> GDNQDRTVANTQPSGPSNSKEIPALTAVETGHTSQVDPSDTLQTRHVVNFHSRSESTVENFMGRAACVFMDQYKLNGEETSTDNFAVWTINVREMAQLRRKCELFTYMRFDIEMTMVITSCQDQGTQLEQDMPVLTHQIMYVPPGGPIPAKVDSYEWQTSTNPSVFWTEGNAPARMSIPFISVGNAYSLFYDGWSHFTQDGTYGYTTLNAMGKLFVRHVNKSSPHQITSTIRVYFKPKHIKAWVPRP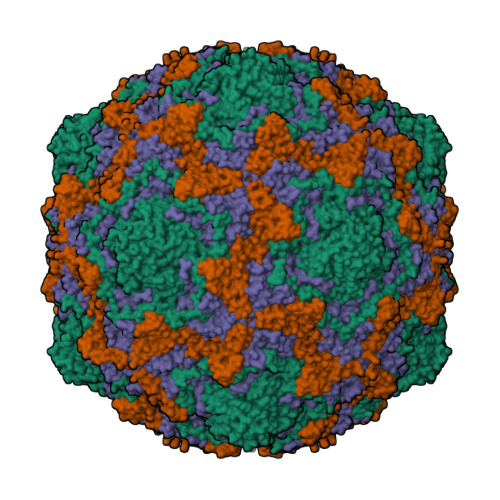PRLCPYINKGDVNFVVTEVTDARKSITDTPH;> SPSAEECGYSDRVRSMTLGNSTITTQESANVVVGYGEWPSYLSDKEATAEDQPTQPDVATCRFYTLESVQWEKSSPGWWWKFPEALKNMGLFGQNMHYHYLGRAGYTIHVQCNASKFHQGCLLVVCVPEAEMGCADTSTTFPATELTTEEEPHVFTSDSITGKKVQAAVCNAGMGVGVGNLTIFPHQWINLRTNNSATIVMPYINSVPMDNMFRHYNFTLMIIPFAPLNFNEGATAYVPVTVTIAPMYAEYNGLRLASTQ;> GVPVLNTPGSTQFLTSDDFQSPSAMPQFDETPEMHIPGEVRNLMEMAEVDSVVPVNNITGKTKSMEAYQIAVGTGNTDKTKPIFSFQMDPGYSSVLKRTLLGEMLNYYAHWSGSVKLTFLFCGSAMATGKLLISYSPPGASVPSSRKDAMLGTHIIWDIGLQSSCVLCVPWISQSHYRMVQQDPYTSAGYITCWYQTNIVVPPGAPTSCDVLCFASACNDFSVRLLRDTPFMAQPGKLQ;> MGAQVSTQKTGAHETSLNAKGNSIIHYTNINFYKDAASSASNRQELQQDPGKFTDPVKDLMVKTLPALN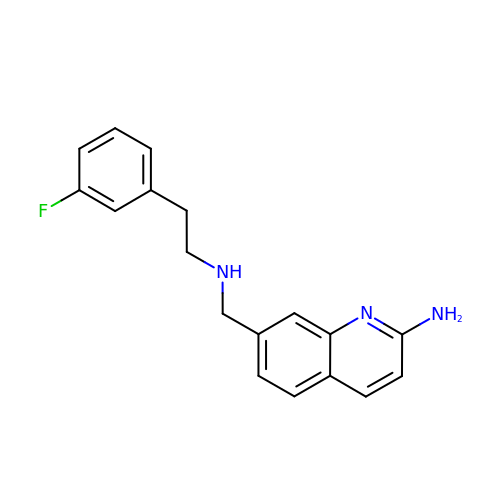7-[[2-(3-fluorophenyl)ethylamino]methyl]quinolin-2-amine | C18 H18 F N3 | YXSBPQQVHVXHJN-UHFFFAOYSA-N>[4x]GSAMTVAYIAIGSNLASPLEQVNAALKALGDIPESHILTVSSFYRTPPLGPQDQPDYLNAAVALETSL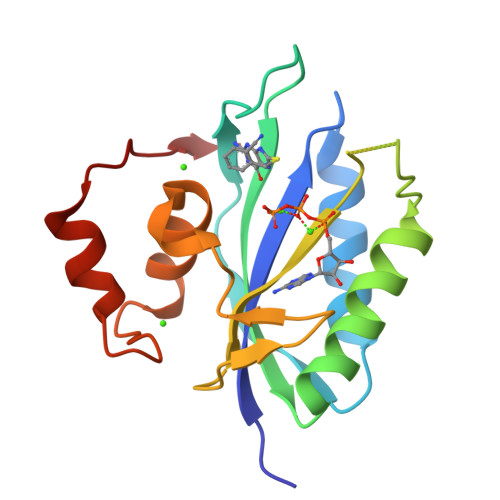APEELLNHTQRIELQQGRVRKAERWGPRTLDLDIMLFGNEVINTERLTVPHYDMKNRGFMLWPLFEIAPELVFPDGEMLRQILHTRAFDKLNKW>[2x]MSTAETAVAPVDYRTDPSQYKHWKLSFNGPVATLGIDIAEDGGIRDGYKLKLNSYDLGVDIELHDAIQRIRFEHPEVRTVVLTSLKDRVFCSGANIFMLGLSTHAWKVNFCKFTNETRNGLEDSSRHSGLKFLAAVNGACAGGGYELALACDEIYLVDDRSSSVSLPEVPLLGVLPGTGGLTRVTDKRKVRHDRADIFCTVVEGVRGERAKAWRLVDEVVKPNQFDQAIQARALELAAQSD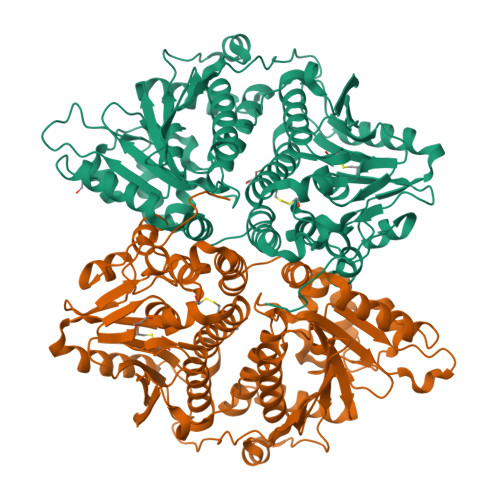RPAHAQGVPLTRIERTDREDGLTYKTLDVTIDRAKRIATFTAKAPQTEPPASIDAIVAAGANWWPLKFAREFDDAILSMRTNELAVGTWVFRTEGDARHLLAADASLMQHKDHWFVRETIGLLRRTLARIDVSSRSLFALIEPGSCFAGTFAELAFAADRTYMAALPANEDEEPAITLSEVNFGLYPMVTHQSRLARRFYEETEPLDAVRSRIGQAIKPVEAERLGLVTASPDDIDWADEIRIALEERAAMSPDALTGLEANLRFNGPETMETRIFGRLTAWQNWIFNRPNAVGEKGALKVYGKGSKAQFDVSRV>MSSVTWAPGNYPSTRRSDHVDTYQSASKGEVPVPDPYQWLEESTDEVDKWTTAQADLAQSYLDQNADIQKLAEKFRASRNYAKFSAPTLLDDGHWYWFYNRGLQSQSVLYRSKEPALPDFSKGDDNVGDVFFDPNVLAADGSAGMVLCKFSPDGKFFAYAVSHLGGDYSTIYVRSTSSPLSQASVAQGVDGRLSDEVKWFKFSTIIWTKDSKGFLYQRYPARERHEGTRSDRNAMMCYHKVGTTQEEDIIVYQDNEHPEWIYGADTSEDGKYLYLYQFKDTSKKNLLWVAELDEDGVKSGIHWRKVVNEYAADYNIITNHGSLVYIKTNLNAPQYKVITIDLSKDEPEIRDFIPEEKDAKLAQVNCANEEYFVAIYKRNVKDEIYLYSKAGVQLTRLAPDFVGAASIANRQKQTHFFLTLSGFNTPGTIARYDFTAPETQRFSILRTTKVNELDPDDFESTQVWYESKDGTKIPMFIVRHKSTKFDGTAAAIQYGYGGFATSADPFFSPIILTFLQTYGAIFAVPSIRGGGEFGEEWHKGGRRETKVNTFDDFIAAAQFLVKNKYAAPGKVAINGAANGGLLVMGSIVRAPEGTFGAAVPEGGVADLLKFHKFTGGQAWISEYGNPSIPEEFDYIYPLSPVHNVRTDKVMPATLITVNIGDGRVVPMHSFKFIATLQHNVPQNPHPLLIKIDKSWLGHGMGKPTDKNVKDAADKWGFIARALGLELKTVE[4x];>MFDTNATRLPIWGIGCNPWTAEHVDQTLASGNDIC[4x]

GmPOPB is the macrocyclase responsible for macrocyclization of amatoxins, eight amino-acid ribosomal peptides with the core sequence IWGIGC(N/D)P. Amatoxins are cyclic peptides further modified by a characteristic sulfoxide cross-link between tryptophan and a cysteine, and hydroxylation (the extent of which vary). GmPOPB is an unusual enzyme catalyzing, depending on substrate length, proteolysis, or macrocyclization using the same catalytic machinery. The protein contains two domains as observed in other POP enzymes. The domain containing the putative catalytic residues (Ser577, Asp661, His698) comprises residues 1–81 and 450–728, and the other domain is a seven bladed β-propeller, comprising residues 82–449.

GmPOPB-S577A (the higher resolution of the pair) bound to the full-length substrate (35mer) belongs to space group P21 with four monomers in the asymmetric unit. For ease of discussion, we split the 35mer into four regions, the 10 residue leader (residues 1–10), the 8 residue core, 6 residue linker, and the 11 residue recognition tail. In all 35mer and 25mer complexes, the enzyme adopts the same “closed” conformation in which the lid (the propeller domain) sits on top of the catalytic domain. In both 25mer complexes the N-terminal residues of the substrate (IWGIGCN) are disordered; in the S577A–35mer complex the N-terminal two residues (MF) are missing, while in the H698A complex only the first N-terminal residue is absent. There are no large differences between the protein backbone positions in the complexes with the 35mer and 25mer substrates (root mean square deviation (rmsd) of 0.48 Å over 720 Cα positions for the S577A structures). Substrate P10, the site of proteolytic cleavage, is positioned for attack by Ser577 (the Cβ of the mutated residue is 3.3 Å from the carbonyl with plausible geometry). Tyr496 is on the opposite face of the carbonyl 2.8 Å from the oxygen and positioned to stabilize the tetrahedral intermediate from attack of Ser577. In the 35mer complex structures, residues 2–9 adopt a helical arrangement that ends up exposed to solvent at the N-terminus and makes few contacts with the protein. In the 35mer complex, the core and linker adopt a tightly packed arrangement that is wedged between the active site loops. We propose the arrangement of and interactions between C-terminal 25 residues and protein that are seen in the 35mer complex act as a kinetic trap, which can only be escaped by dissociation.>[2x]MNPSKSISRVAQELSKYEILKKLDESDTESYSSVYLCKKKGEHKRFVCKIVKPSTFNSLEFDVHILMRNNPNFIKLHNFVFNDNGESLLIMDYVSDGDLFDFVKMNDTRELR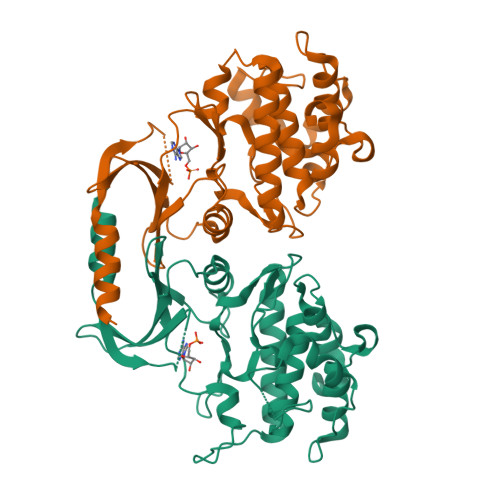LNEAACKKIIITLVTALNDLHKNNIVHNDVKLENLLYDRKKKRLFVCDYGLSRIVGTPSFYDGTTVYFSPEKIRHEAYQTSFDWWAVGVVAYEILSTEYPFDINEDNEEEMDAIEPKDMLPLYSKPLPTIEHVSKKANDFVRRMLALDINSRLSTYDEIIKHPFLCF>[5x]MPSKKNGRSGPQPHKRWVFTLNNPSEDERKKIRDLPISLFDYFIVGEEGNEEGRTPHLQGFANFVKKQTFNKVKWYLG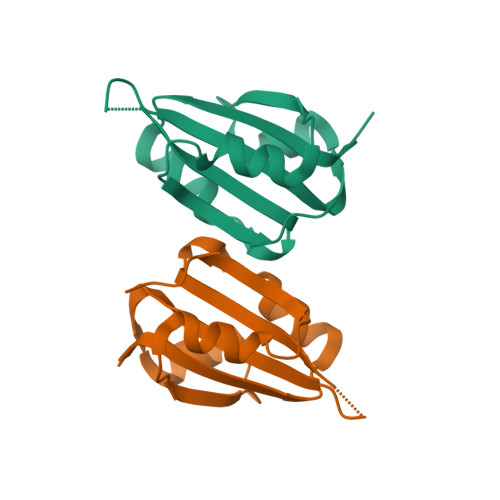ARCHIEKAKGTDQQNKEYCSKEGNLLIECGAPRSQGQRSDLSTAVSTLLESGSLVTVAEQHPVTFVRNFRGLLEHHHHHH> SVNNSQLVVSVAGTVEGTNQDISLKFFEIDLTSRPAHGGKTEQGLSPKSKPFATDSGAMPHKLEKADLLKAIQEQLIANVHSNDDYFEVIDFASDATITDRNGKVYFADKDGSVTLPTQPVQEFLLSGHVRVRPYKEKPIQNQAKSVDVEYTVQFTPLNPDDDFRPGLKDTKLLKTLAIGDTITSQELLAQAQSILNKTHPGYTIYERDSSIVTHDNDIFRTILPMDQEFTYHVKNREQAYEINKKSGLNEEINNTDLISEKYYVLKKGEKPYDPFDRSHLKLFTIKYVDVNTNELLKSEQLLTASERNLDFRDLYDPRDKAKLLYNNLDAFGIMDYTLTGKV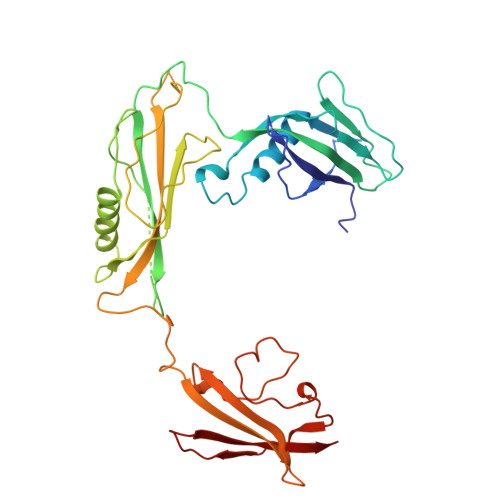EDNHDDTNRIITVYMGKRP>[2x]WKEIKFEFDTIDPADSFSGASPERKAAVALRSLFTFVAARVVLEQLQGPGGPETTYNQQAYLDLMDFLGTPMKGDGGDEWMAAVMRKNHALALRLMEVREAYLDEFEWGKTMEMASRET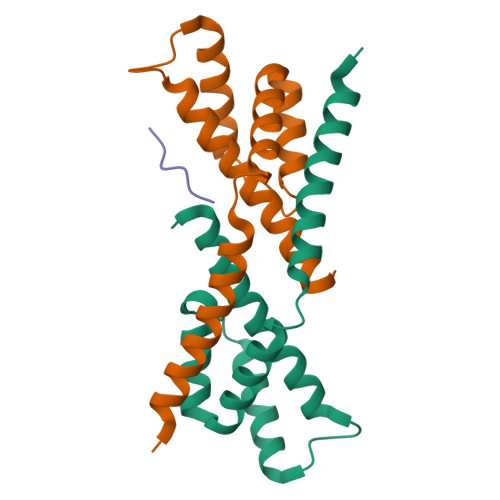REANTRLMRAAAM;> WKEIKF~{N}-[3-(7,8-dihydro-5~{H}-[1,3]dioxolo[4,5-g]isoquinolin-6-ylmethyl)phenyl]-2-ethyl-2-methanoyl-butanamide 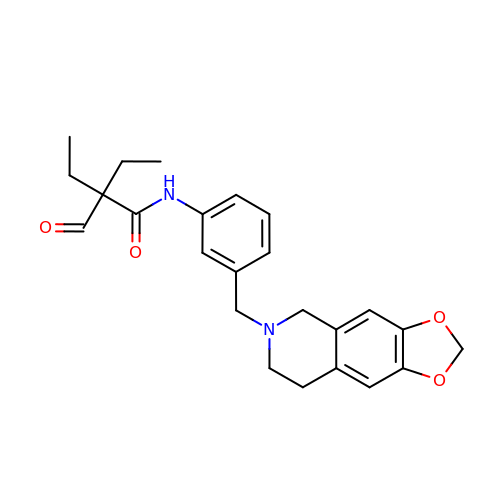| C24 H28 N2 O4 | DZOGMSIEUICIFK-UHFFFAOYSA-N>YSQTKADVVWKDVDGVSMPIPPKTHPRLYLREQQVPDLKNRMNDPKLKKVWADMIKMQEDWKPADIPEVKDFRFYFNQKGLTVRVELMALNYLMTKDPKVGREAITSIIDTLETATFKPAGDISRGIGLFMVTGAIVYDWCYDQLKPEEKTRFVKAFVRLAKMLECGYPPVKDKSIVGAASEWMIMRDLLSVGIAIYDEFPEMYNLAAGRFFKEHLVARNWFYPSHNYHQGMSALNVRFTNDLFALWILDRMGAGNVFNPGQQFILYDAIYKRRPDGQILAGGDVDYSRKKPKYYTMPALLAGSYYKDEYLNYEFLKDPNVEPHCKLFEFL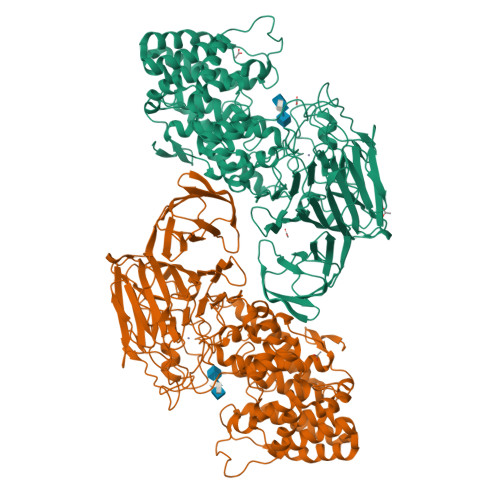WRDTQLGSRKPDDLPLSRYSGSPFGWMIARTGWGPESVIAEMKVNEYSFLNHQHQDAGAFQIYYKGPLAIDAGSYTGSSGGYNSPHNKNFFKRTIAHNSLLIYDPKETFSSSGYGGSDHTDFAANDGGQRLPGKGWIAPRDLKEMLAGDFRTGKILAQGFGPDNQTPDYTYLKGDITAAYSAKVKEVKRSFLFLNLKDAKVPAAMIVFDKVVASNPDFKKFWLLHSIEQPEIKGNQITIKRTKNGDSGMLVNTALLPDAANSNITSIGGKGKDFWVFGTNYTNDPKPGTDEALERGEWRVEITPKKAAAEDYYLNVIQIADNTQQKLHEVKRIDGDKVVGVQLADRIVTFSKTSETVDRPFGFSVVGKGTFKFVMTDLLPGTWQVLKDGKILYPALSAKGDDGALYFEGTEGTYRFLR[2x]>MIRTMLQGKLHRVKVTHADLHYEG[2x];>[2x]XCAIDQDFLDAAGILENEAIDIWNVTNGKRFSTYAIAAERGSRIISVNGAAAHCASVGDI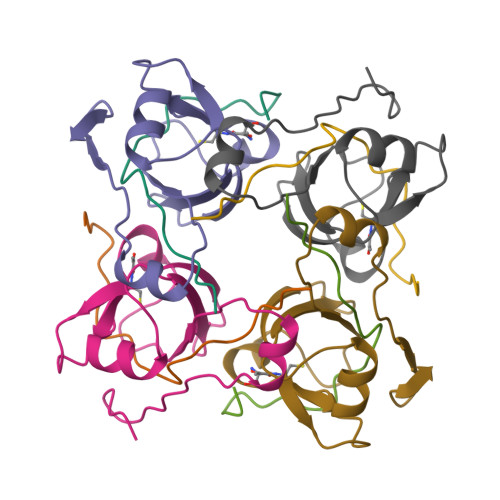VIIASFVTMPDEEARTWRPNVAYFEGDNEMK> GSEGHRTLASTPALWASIPCPRSELRLDLVLPSGQSFRWREQSPAHWSGVLADQVWTLTQTEEQLHCTVYRGDKSQASRPTPDELEAVRKYFQLDVTLAQLYHHWGSVDSHFQEVAQKFQGVRLLRQDPIECLFSFICSSNNNIARITGMVERLCQAFGPRLIQLDDVTYHGFPSLQALAGPEVEAHLRKLGLGYRARYVSASARAILEEQGGLAWLQQLRESSYEEAHKALCILPGVGTKVADCICLMALDKPQAVPVNVHMWHIAQRDYSWHPTTSQAKGPSPQTNKELGNFFRSLWG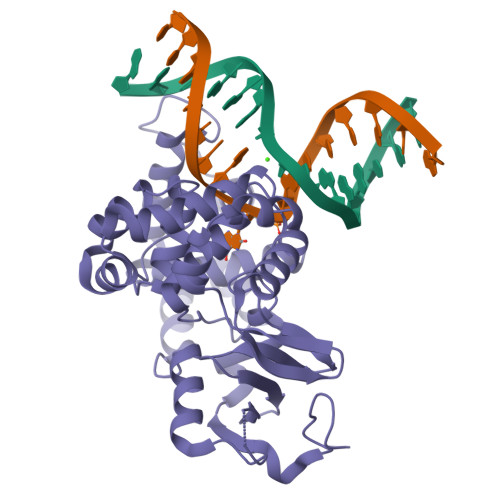PYAGWAQAVLFSADLRQ2-({2-[(3R)-3-aminopiperidin-1-yl]-5-bromo-6-oxopyrimidin-1(6H)-yl}methyl)benzonitrile | C17 H18 Br N5 O | 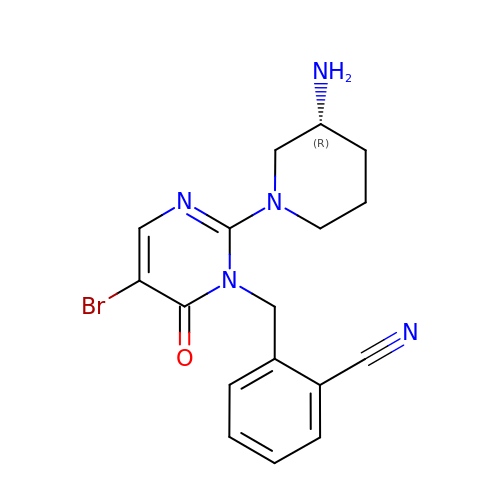GGCILSXUAHLDMF-CQSZACIVSA-N>[2x]GGGGGPDYLYAEYRALPSPRQTGKNLRIGDGFSKYDNMTGVYLEKGRHVVLVGKTEGQEISLLLPNLMRKPAEGVQPTKDPNGWGLHKKQIPLKEGINIIDVETPANAYISYFTEDAGKAPKIPVHFVTGKANGYFDTTRGDTNKDWVRLLDQAVSPIMDARGKYIQVAYPVEFLKKFTKDRGTELINAYDKLIGIQYQLMGLDKYG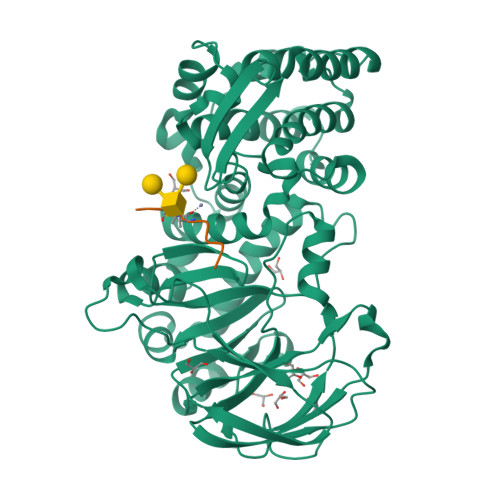KIPENRVLARVNFNYYMFRDGDGVAYLGNDGTMRMVTDPENVLKGDACWGFSHAVGHVMQMRPMTWGGMTEVSNNIFSLQAAAKTGNESRLKRQGSYDKARKEIIEGEIAYLQSKDVFNKLVPLWQLHLYFTKNGHPDFYPDVMEYLRNNAGNYGGNDTVKYQFEFVKACCDVTKTDLTDFFEKWGFFKPGKFHIGDYAQYDFNVTPEMVEETKKWIAGKGYPKPETDITELSE;>TEAQTTPPPA[2x]> QGMSTFGSVFRVTTYGESHCKSVGCIVDGCPPGLELTEADIQPQLSRRRPGQSALSTPRNEKDQVQIQSGTEHGKTLGSPIGMMVMNQDHRPGDYSETDLYPRPSHADWTYMQKYGVKSASGGGRSSARETIGRVAAGAIAEKILKKANNVEIVAFVSSIGEVSMDRNPQDAKFQQLLNTITREEVDSVGPIRCPDPEVREQMVKVIEKYRDAKDSIGGVVTCVIRNCPVGLGEPCFDKLEATLAHAMMSLPATKGFEFGSGFAGTRIPGSKHNDPFYFSEEDQRLRTKTNNSGGVQGGISNGENIYFSVAFKSAATISQEQETSTYDGKDGVLAARGRHDPSVTPRAVPIVES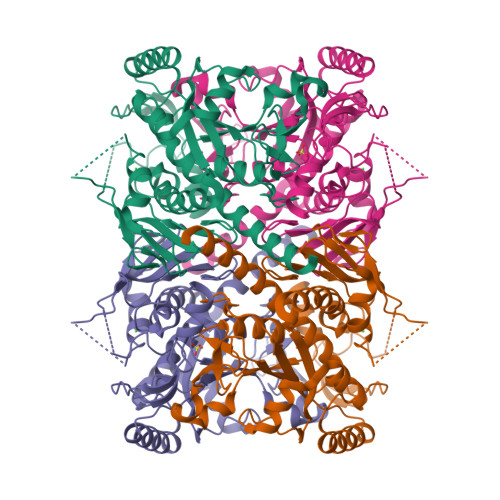MAALVLVDQLLIQKSREYGKSIVA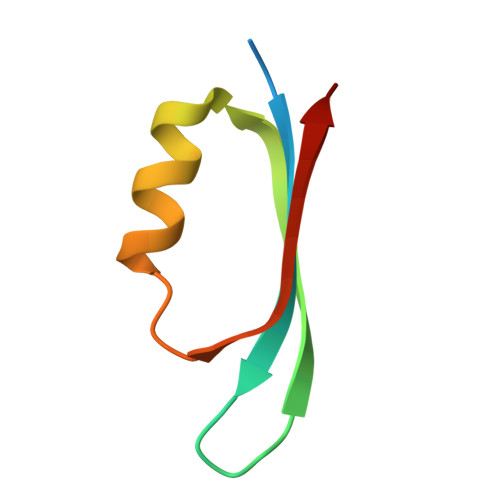> MVQNDFVDSYDVTMLLQDDDGKQYYEYHKGLSLSDFEVLYGNTADEIIKLRLDKVL>[12x]GPGFLPSFQHFATQAIHVGQEPEQWSSRAVVLPISLATTFKQDSPGQSSGFVYSRSGNPTRNCLEKAVAALDGAKHCLTFASGLAATTTITHLLKAGDEVICMDEVYGGTNRYFRRVASEFGLKISFVDCSKTKLLEAAITPQTKLVWIETPTNPTLKLADIK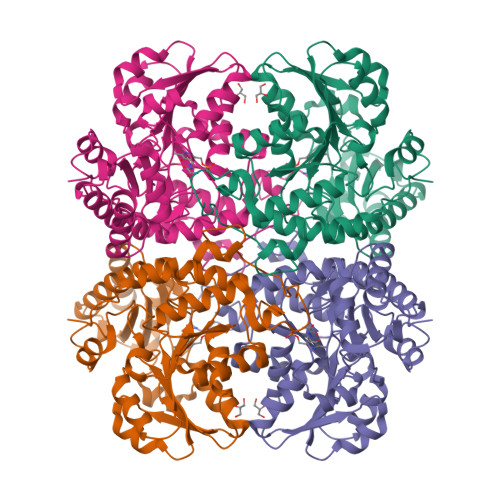ACAQIVHKHKDIILVVDNTFMSAYFQRPLALGADICMCSATKYMNGHSDVVMGLVSVNSDDLNERLRFLQNSLGAVPSPFDCYLCCRGLKTLQIRMEKHFRNGMAVARFLESNPRVEKVIYPGLPSHPQHELAKRQCTGCPGMVSFYIKGTLQHAQVFLKNIKLFALAESLGGYESLAELPAIMTHASVPEKDRATLGISDTLIRLSVGLEDEKDLLEDLGQALKAAHP> GSSDPNEAV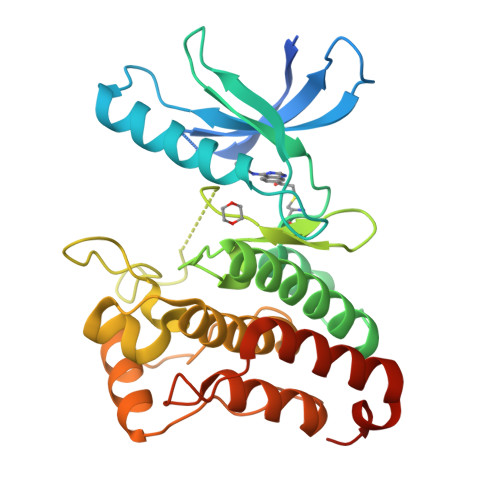REFAKEIDVSCVKIEEVIGAGEFGEVCRGRLKQPGRREVFVAIKTLKVGYTERQRRDFLSEASIMGQFDHPNIIRLEGVVTKSRPVMILTEFMENCALDSFLRLNDGQFTVIQLVGMLRGIAAGMKYLSEMNYVHRDLAARNILVNSNLVCKVSDFGLSRFLEDDPSDPTYTSSLGGKIPIRWTAPEAIAYRKFTSASDVWSYGIVMWEVMSYGERPYWDMSNQDVINAVEQDYRLPPPMDCPTALHQLMLDCWVRDRNLRPKFSQIVNTLDKLIRNPASLKVIASAQS>MEQALNRVITKIRQVSDLESIFSTTTQEVRRLFGIE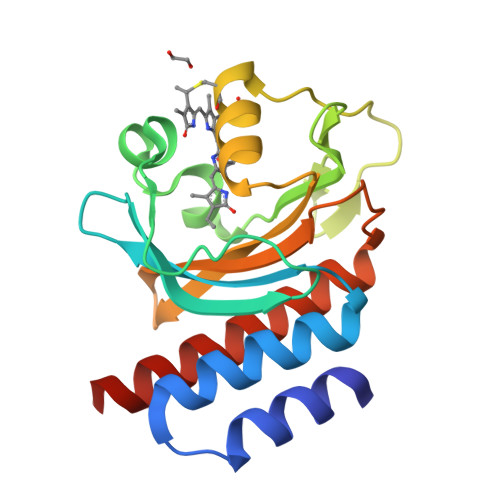RVTIYKFREDYFGDFITESEAGGWRKLVGSGWEDPYLNEHQGGRFQQNQPFVVDDIYLGETIWEEGKFNLQKPKRPLTDCHIEALESFEVKSCAVVAIFQGQKLWGLLSAFQNSAPRHWDEAEVQLLMRVADQLGVAIQQAEYLAQ[2x]> MKIEFDVVVVGAGPSGLSCAYVLAKNGLKVAVVEKGEYPGSKNVMGGVLYVHPLKEIMP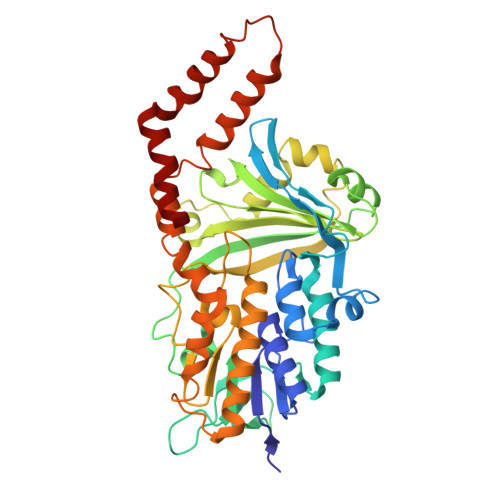DFLEKAANSKALERNVIEQNLWLLGNEGVIKIGHRNVEWKENPNAFTVLRANFDRWFAQEVEKAGALIIPKTKVEDFLRNEKGEIAGVVTSRPKGEIHSKAVVIAEGVNPILTMKAGLRKEDLKPHMVAVAVKEVISVPEDVVNRVFGVEGNDGATIELLGSWSEGMFGMGFLYANRSSVSLGCGVLLEDLRKKKIKPYQLLENLKNHPVISDMLGEYRNNTMEYLAHLIPEGGYYAMPKVYGDRVLVCGDAAMLVNSIHREGSNHAITSGRLAAETLLEAFEKGDFSEKILKNYYLRLKESFILKDLEKYKDLMPTMEKNHQFVEIYPDLANDALKRFLQVDGTPKWDVQKQIADMVLSRRSLIGISLDLLRFWRAVR> MDSTSTIANKIEEYLGAKSDDSKIDELLKADPSEVEYYRSGGDGDYLKNNICKITVNHSDSGKYDPCEKKLPPYDDNDQWKCQQNSSDGSGKPENICVPPRRERLCTYNLENLKFD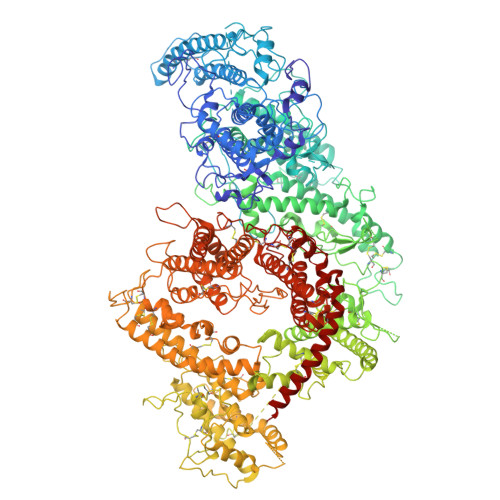KIRDNNAFLADVLLTARNEGEKIVQNHPDTNSSNVCNALERSFADLADIIRGTDQWKGTNSNLEKNLKQMFAKIRENDKVLQDKYPKDQKYTKLREAWWNANRQKVWEVITCGARSNDLLIKRGWRTSGKSDRKKNFELCRKCGHYEKEVPTKLDYVPQFLRWLTEWIEDFYREKQNLIDDMERHREECTREDHKSKEGTSYCSTCKDKCKKYCECVKKWKTEWENQENKYKDLYEQNKNKTSQKNTSRYDDYVKDFFEKLEANYSSLENYIKGDPYFAEYATKLSFILNPSDGILQENCSDNKRGSSSNDSCDNKNQDECQKKLEKVFASLTNGYKCDKCKSGTSRSKKKWIWKKSSGNEEGLQEEYANTIGLPPRTQSLYLGNLPKLENVCEDVKDINFDTKEKFLAGCLIVSFHEGKNLKKRYPQNKNSGNKENLCKALEYSFADYGDLIKGTSIWDNEYTKDLELNLQNNFGKLFGKYIKKNNTAEQDTSYSSLDELRESWWNTNKKYIWTAMKHGAEMNITTCNADGSVTGSGSSCDDIPTIDLIPQYLRFLQEWVENFCEQRQAKVKDVITNCKSCKESGNKCKTECKTKCKDECEKYKKFIEACGTAGGGIGTAGSPWSKRWDQIYKRYSKHIEDAKRNRKAGTKNCGTSSTTNAAASTDENKCVQSDIDSFFKHLIDIGLTTPSSYLSNVLDDNICGADKAPWTTYTTYTTTEKCNKERDKSKSQSSDTLVVVNVPSPLGNTPYRYKYACQCKIPTNEETCDDRKEYMNQWSCGSARTMKRGYKNDNYELCKYNGVDVKPTTVRSNSSKLDGNDVTFFNLFEQWNKEIQYQIEQYMTNANISCIDEKEVLDSVSDEGTPKVRGGYEDGRNNNTDQGTNCKEKCKCYKLWIEKINDQWGKQKDNYNKFRSKQIYDANKGSQNKKVVSLSNFLFFSCWEEYIQKYFNGDWSKIKNIGSDTFEFLIKKCGNNSAHGEEIFSEKLKNAEKKCKENESTDTNINKSETSCDLNATNYIRGCQSKTYDGKIFPGKGGEKQWICKDTIIHGDTNGACIPPRTQNLCVGELWDKSYGGRSNIKNDTKELLKEKIKNAIHKETELLYEYHDTGTAIISKNDKKGQKGKNDPNGLPKGFCHAVQRSFIDYKNMILGTSVNIYEHIGKLQEDIKKIIEKGTPQQKDKIGGVGSSTENVNAWWKGIEREMWDAVRCAITKINKKNNNSIFNGDECGVSPPTGNDEDQSVSWFKEWGEQFCIERLRYEQNIREACTINGKNEKKCINSKSGQGDKIQGACKRKCEKYKKYISEKKQEWDKQKTKYENKYVGKSASDLLKENYPECISANFDFIFNDNIEYKTYYPYGDYSSICSCEQVKYYKYNNAEKKNNKSLCYEKDNDMTWSKKYIKKLENGRSLEGVYVPPRRQQLCLYELFPIIIKNEEGMEKAKEELLETLQIVAEREAYYLWKQYNPTGKGIDDANKKACCAIRGSFYDLEDIIKGNDLVHDEYTKYIDSKLNEIFGSSNTNDIDTKRARTDWWENETITNGTDRKTIRQLVWDAMQSGVRYAVEEKNENFPLCMGVEHIGIAKPQFIRWLEEWTNEFCEKYTKYFEDMKSKCDPPKRADTCGDNSNIECKKACANYTNWLNPKRIEWNGMSNYYNKIYRKSNKESEDGKDYSMIMAPTVIDYLNKRCHGEINGNYICCSCKNIGAYNTTSGTVNKKLQKKETECEEEKGPLDLMNEVLNKMDKKYSAHKMKCTEVYLEHVEEQLNEIDNAIKDYKL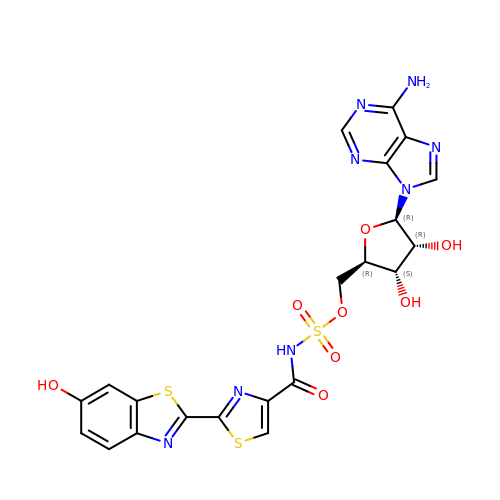5'-O-[N-(DEHYDROLUCIFERYL)-SULFAMOYL] ADENOSINE | C21 H18 N8 O8 S3 | LJLYTUYNVSHXQB-SOONXTGKSA-N> GSEGHRTLASTPALWASIPCPRSELRLDLVLPSGQSFRWREQSPAHWSGVLADQVWTLTQTEEQLHCTVYRGDKSQASRPTPDELEAVRKYFQLDVTLAQLYHHWGSVDSHFQQVAQKFQGVRLLRQDPIECLFSFICSSNNNIARITGMVERLCQAFGPRLIQLDDVTYHGFPSLQALAGPEVE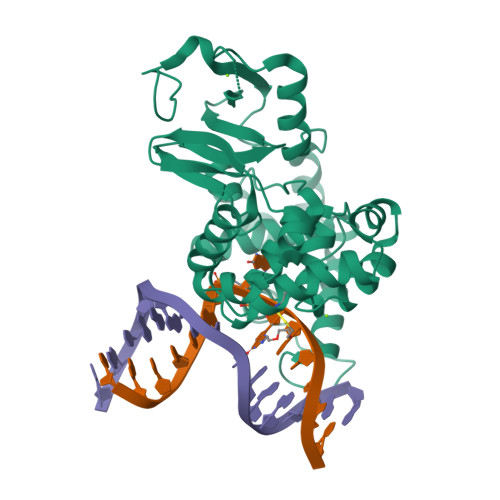AHLRKLGLGYRARCVSASARAILEEQGGLAWLQQLRESSYEEAHKALCILPGVGTQVADCICLMALDKPQAVPVDVHMWHIAQRDYSWHPTTSQAKGPSPQTNKELGNFFRSLWGPYAGWAQAVLFSADLRQ[4-(1H-benzimidazol-1-yl)phenyl]methanol 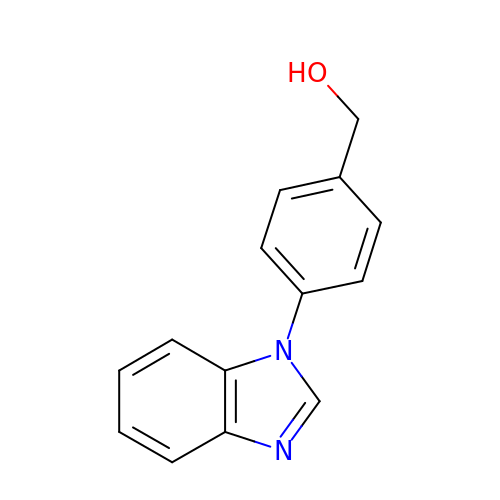| C14 H12 N2 O | IRZKUEWQJPIBJF-UHFFFAOYSA-N N~3~-{(1S,2R)-1-(3,5-DIFLUOROBENZYL)-2-HYDROXY-3-[(3-METHOXYBENZYL)AMINO]PROPYL}-N~1~,N~1~-DIPROPYLBENZENE-1,3,5-TRICARBOXAMIDE 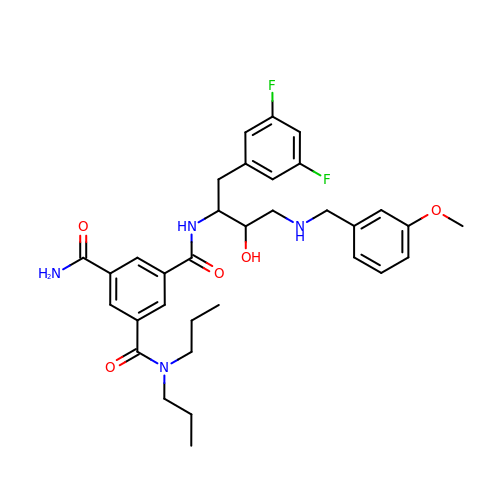| C33 H40 F2 N4 O5 | XIQAKRFMIYGAIR-XZWHSSHBSA-N>U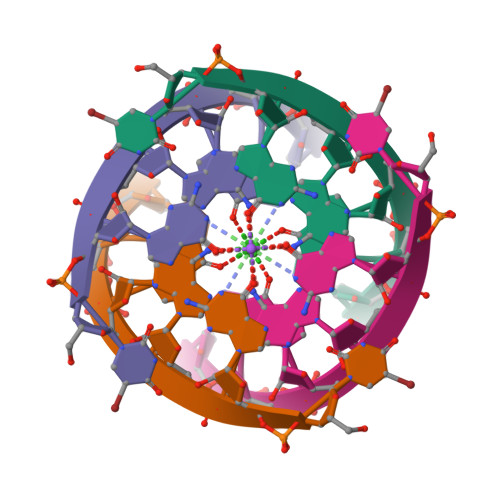GAGGU[4x]> LPTSNPAQELEARQLERTTRDDLINGNSASCADVIFIYARGSTETGNLGTLGPSIASNLESAFGKDGVWIQGVGGAYRATLGDNALPRGTSSAAIREMLGLFQQANTKCPDATLIAGGYSQGAALAAASIEDLDSAIRDKIAGTVLFGYTKNLQNRG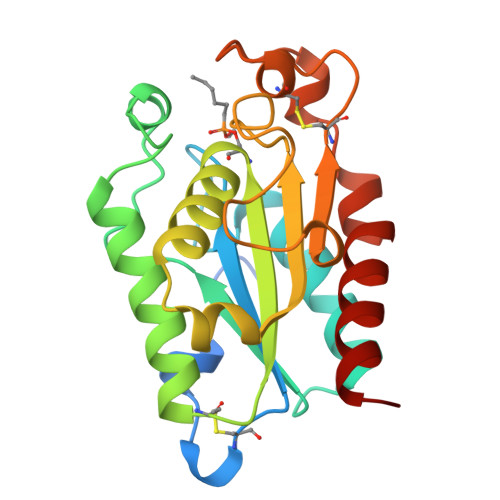RIPNYPADRTKVFCNTGDLVCTGSLIVAAPHLAYGPDARGPAPEFLIEKVRAVRGSA>[2x]GIDPFTMNAKPGFTDYIVKDIALADFGRKEISLAETEMPGLMATREEYGPKQPLKGARIAGSLHMTIQTAVLIETLAALGADIRWVSCNIYSTQDHAAAAIAAAGIPVFAVKGETLTEYWDYTAKLFDWHGGGTPNMILDDGGDATMLVHAGYRAEQGDTAFLDKPGSEEEEIFYALVKRLLKEKPKGWFAEIAKNIKGVSEETTTGVHRLYEMANKGTLLFPAINVNDSVTKSKFDNLYGCRESLVDGIRRGTDVMLSGKVAMVAGFGDVGKGSAASLRQAGCRVMVSEVDPICALQAAMEGYEVVTMEDAAPRADIFVTATGNKDIITIEHMRAMKDRAIVCNIGHFDNEIQIASLRNLKWTNIKPQVDEIEFPDKHRIIMLSEGRLVNLGNAMGHPSFVMSASFTNQTLAQIELFANNKDSKYAKKVYVLPKTLDEKVARLHLAKIGVKLTELRKDQADYIGVKQEGPYKSDHYRY

SAH, which is formed upon methyl-group transfer from SAM, must be removed from the reaction equilibrium (which is shifted far towards SAH formation) by its hydrolase (SAHase; De La Haba & Cantoni, 1959), which splits it into Ado and homocysteine (Hcy). In this way, SAHase is a key regulator of SAM-dependent methylation reactions and of Hcy levels, which, when elevated, are a risk factor for neurodegenerative diseases, neural tube defects and cardiovascular diseases. A typical SAHase protomer is usually divided into three closely connected domains: an N-terminal substrate-binding domain, a cofactor-binding domain and a small C-terminal dimerization domain. The substrate-binding and cofactor-binding domains are separated by a bipartite hinge, allowing them to oscillate between two conformational states, closed and open, during the catalytic cycle.

Only the Ade complex crystallized with a dimer in the asymmetric unit, while all of the other complexes formed a crystallographically independent tetrameric assembly. The incubation of ligand-free BeSAHase (§2.2.2) with Ade resulted in crystals with a dimer in the asymmetric unit, from which the complete tetramer is created by crystallographic symmetry. The first four residues of chain A and the first five residues of chain B are not visible in electron density. In each subunit, one Ade molecule is found in the active site, accompanied by a sodium cation. Also, one NAD+ cofactor molecule is found in each protomer. Moreover, 570 water molecules, plus two bromide anions and five ethylene glycol molecules from the crystallization buffer, were modelled in the electron density of the solvent region. Ade molecules were found in two structures. In both structures, despite the absence of the sugar moiety, the architecture of the active site is preserved, as observed previously by Brzezinski et al.. In a pattern of molecular mimicry, four water molecules imitate the positions of the O2′, O3′, O4′ and O5′ atoms of an Ado molecule and create hydrogen bonds to the corresponding side-chain atoms of the protein.> MGRSHHHHHHGSLVPRGSEQGSNVNHLIKVTDQSITEGYDDSDGIIKAHDAENLIYDVTFEVDDKVKSGDTMTVNIDKNTVPSDLTDSFAIPKIKDNSGEIIATGTYDNTNKQITYTFTDYVDKYENIKAHLKLTSYIDKSKVPNNNTKLDVEYKTALSSVNKTITVEYQKPNENRTANLQSMFTNIDTKNHTVEQTIYINPLRYSAKETNVNISGNGDEGSTIIDDSTIIKVYKVGDNQNLPDSNRIYDYSEYEDVTN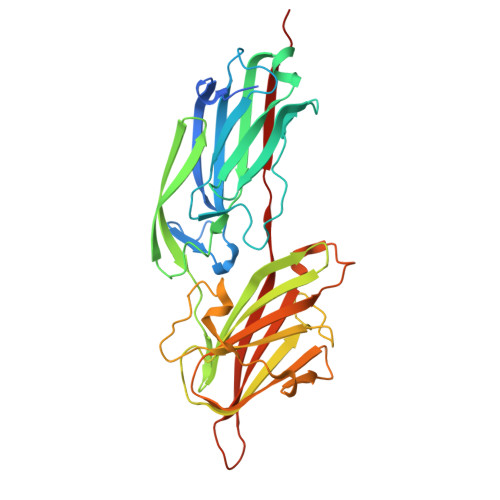DDYAQLGNNNDVNINFGNIDSPYIIKVISKYDPNKDDYTTIQQTVTMQTTINEYTGEFRTASYDNTIAFSTSSGQGQGDLPPEK~{N}-(3-chlorophenyl)-4-methyl-3-[(1-methyl-6-pyridin-3-yl-pyrazolo[3,4-d]pyrimidin-4-yl)amino]benzamide 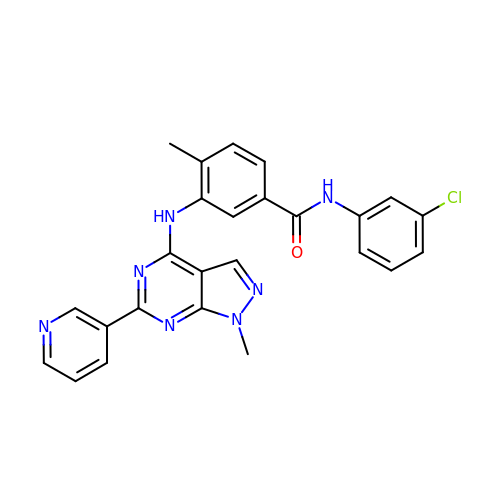| C25 H20 Cl N7 O | VGMNSQKPXFXZPZ-UHFFFAOYSA-N(12~{R})-7-[(4-chlorophenyl)methyl]-12-(ethoxymethyl)-11-[(3-fluorophenyl)methyl]-2,5,7,11-tetrazatricyclo[7.4.0.0^{2,6}]trideca-1(9),5-dien-8-one | C26 H28 Cl F N4 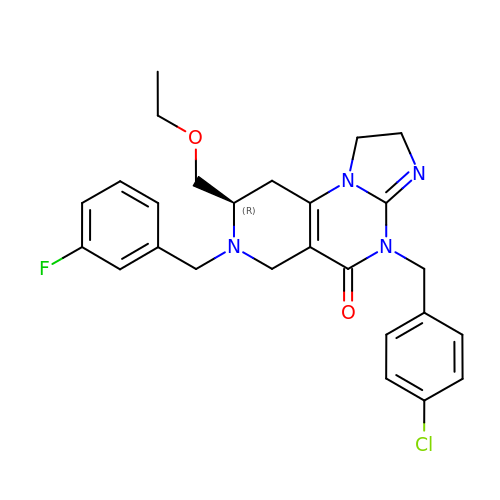O2 | VCPJLNSMEZPNKY-JOCHJYFZSA-N> MAPGCKTELRSVTNGQSNQPSNEGDAIKVFVRIRPPAERSGSADGEQNLCLSVLSSTSLRLHSNPEPKTFTFDHVADVDTTQESVFATVAKSIVESCMSGYNGTIFAYGQTGSGKTFTMMGPSESDNFSHNLRGVIPRSFEYLFSLIDREKEKAGAGKSFLCKCSFIEIYNEQIYDLLDSASAGLYLREHIKKGVFVVGAVEQVVTSAAEAYQVLSGGWRNRRVASTSMNRESSRSHAVFTITIESMEKSNEIVNIRTSLLNLVDLAGSERQKDTHAEGMRLKEAGNINRSLSCLGQVITALVDVGNGKQRHVCYRDSKLTFLLRDSLGGNAKTAIIANVHPGSRCFGETLSTLNFAQRAKLIKNKAVVNEDTQG;> MANVPWAEVCEKFQAALALSRVELHKNPEKEPYKSKYSARALLEEVKALLGPAPEDEDERPEAEDGPGAGDHALGLPAEVVEPEGPVAQRAVRLAVIEFHLGVNHIDTEELSAGEEHLVKCLRLLRRYRLSHDCISLCIQAQNNLGILWSEREEIETAQAYLESSEALYNQYMKEVGSPPLDPTERFLPEEEKLTEQERSKRFEKVYTHNLYYLAQVYQHLEMFEKAAHYCHSTLKRQLEHNAYHPIEWAINAATLSQFYINKLCFMEARHCLSAANVIFGQTGKISATEDTPEAEGEVPELYHQRKGEIARCWIKYCLTLMQNAQLSMQDNIGELDLDKQSELRALRKKELDEEESIRKKAVQFGTGELCDAISAVEEKVSYLRPLDFEEARELFLLGQHYVFEAKEFFQIDGYVTDHIEVVQDHSALFKVLAFFETDMERRCKMHKRRIAMLEPLTVDLNPQYYLLVNRQIQFEIAHAYYDMMDLKVAIADRLRDPDSHIVKKINNLNKSALKYYQLFLDSLRDPNKVFPEHIGEDVLRPAMLAKFRVARLYGKIITADPKKELENLATSLEHYKFIVDYCEKHPEAAQEIEVELELSKEMVSLLPTKMERFRTKMALT

Kinesin-binding protein (KIFBP), which is mutated in Goldberg-Shprintzen syndrome, binds to and inhibits the catalytic motor heads of 8 of 45 kinesin superfamily members, but the mechanism remains poorly defined. KIFBP interacts directly with the motor head of Kinesin-2 (KIF3A), Kinesin-3 (KIF1A, KIF1B, KIF1C, KIF13B, and KIF14), Kinesin-8 (KIF18A), and Kinesin-12 (KIF15) family members, resulting in inhibition of motor-microtubule binding both in vitro and in cells. We show that KIFBP is a tandem repeat protein constructed of nine helix pairs that assemble into a solenoid-like structure. Collectively, our work describes the molecular mechanism of KIFBP-mediated inhibition of KIF15 and KIF18A via binding to and stabilizing a conformation of the kinesin motor head that is incompatible with microtubule binding.

After determining the structure of KIFBP alone, we used cryo-EM to determine the structure of KIFBP bound to KIF15. Unexpectedly, when we docked the structure of KIF15 into the reconstruction, we noticed that the α4 helix of KIF15 was missing. Instead, we noticed the presence of an additional α-helical density within a cleft of KIFBP, suggesting the displacement of KIF15-α4 into this cleft during complex formation. In the structure, KIFBP occupies the microtubule-binding surface of KIF15, sterically blocking access to the microtubules by KIF15. The most notable structural change involved the repositioning of KIF15-α4 away from the kinesin motor domain, placing KIF15-α4 15 Å away from the location found in the crystal structure of KIF15 (37). The adjoining loops on each side of KIF15-α4, Loop-11 (“KIF15-L11”) and Loop-12 (“KIF15-L12”), accommodated the repositioning of KIF15-α4 by facilitating the extension of KIF15-α4 away from the body of the motor domain. Whereas KIF15-L12 remains extended in solution, KIF15-L11 is positioned away from the motor domain and binds along KIFBP-HP4a. In addition to seeing changes in KIF15-L11, KIF15-α4, and KIF15-L12, we saw that the overall structure of KIF15 adopted a more open conformation. The structure showed the shift of α helices KIF15-α1, KIF15-α3, and KIF15-α6 away from the core of the motor. Thus, KIFBP blocks microtubule binding by sterically preventing microtubule interaction in addition to allosterically altering the KIF15 motor.FERULOYL COENZYME A | C31 H44 N7 O20 P3 S | 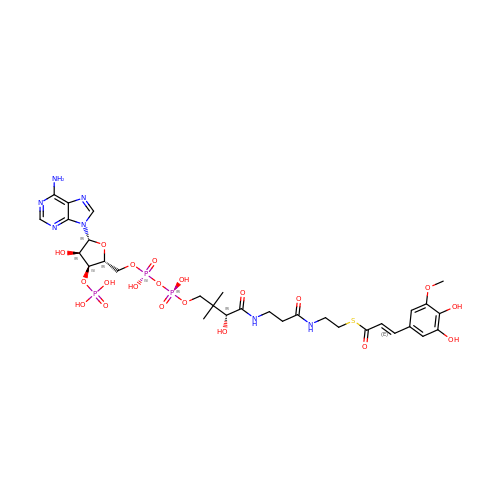ILSPFIPSQSFPCN-VYBUCKLUSA-N> MASWDSPTASSNGDLIEEIQASSTSTDPRTFTGLSIVEDIGDVVPVTDNASPALPVSLTDADGNDVVVEDVSRILPLDLYGTYSKTIAGLGLVDNIVGRTVSSTEPALADTEVVTTGGHTLNAEAILNLHPTLVIIDHSIGPREVIDQIRAAGVATVIMSPQRSIASIGDDIRDIASVVGLPEEGEKLAE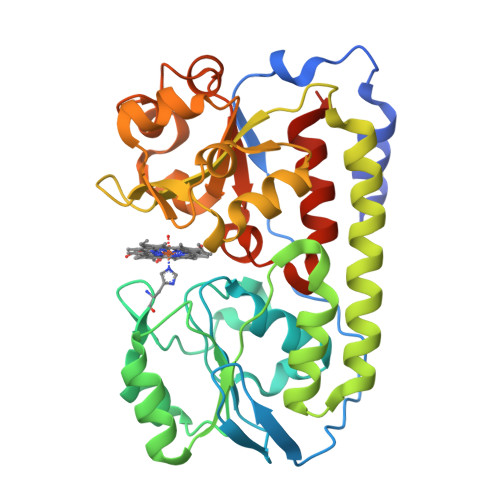RSVAEVEEASTVVDELTPEDPLKMVFLAARGTGGVFFILGDAYGGRDLIEGLGGVDMAAEKGIMDLAPANAEALAELNPDVFVMMSEGLVSTGGIDGLMERPGIAQTTAGQNQRVLALPDGQSLAFGAQTGELLLRASRELYVQGGELEHHHHHH>[2x]VGVSGSAEGFAEGVTGGGDATPVYPDTIDELVSYLGDDEARVIVLTKTFDFTDSEGTTTGTGCAPWGTASACQVAIDQDDWCENYEPDAPSVSVEYYNAGVLGIT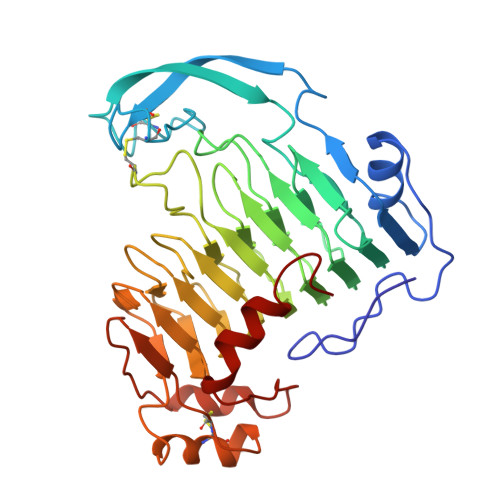VTSNKSLIGEGSSGAIKGKGLRIVSGAENIIIQNIAVTDINPKYVWGGDAITLDDCDLVWIDHVTTARIGRQHYVLGTSADNRVSLTNNYIDGVSDYSATCDGYHYWGIYLDGDADLVTMKGNYIYHTSGRSPKVQDNTLLHCVNNYFYDISGHAFEIGEGGYVLAEGNVFQNVDTVLETYEGAAFTVPSTTAGEVCSTYLGRDCVINGFGCSGTFSEDSTSFLSDFEGKNIASASAYTSVASRVVANAGQGNL>[3x]NDKLTLWTTPDPSPNCKVSEEKDSKLTLVLTKCGSQILASVSLLVVKGKFANINNETNPGEDYKKFS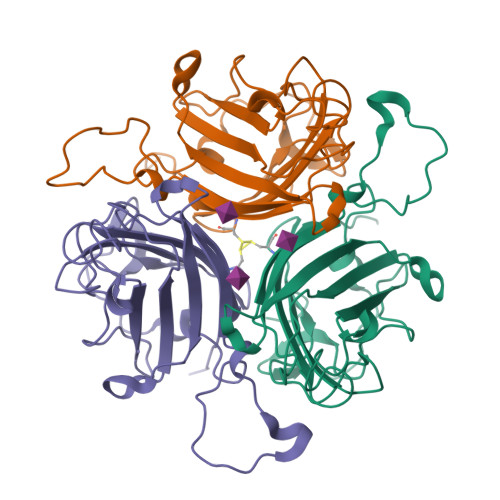VKLLFDANGKLLTGSSLDGNYWNYKNKDSVIGSPYENAVPFMPNSTAYPKIINNGTANPEDKKSAAKKTIVTNVYLGGDAGQPVATTVSFNKETESNCVYSITFDFAWNKTYKNVPFDSSSLTFSYIAQDAEDKNE>[2x]SEFVPPPECPVFEPSWEEFTDPLSFIGRIRPLAEKTGICKIRPPKDWQPPFACEVKSFRFTPRVQRLNELEAMTRVRLDFLDQLAKFWELQGSTLKIPVVERKILDLYALSKIVASKGGFEMVTKEKKWSKVGSRLGYLPGKGTGSLLKSHYERILYPYELFQSGVSLMG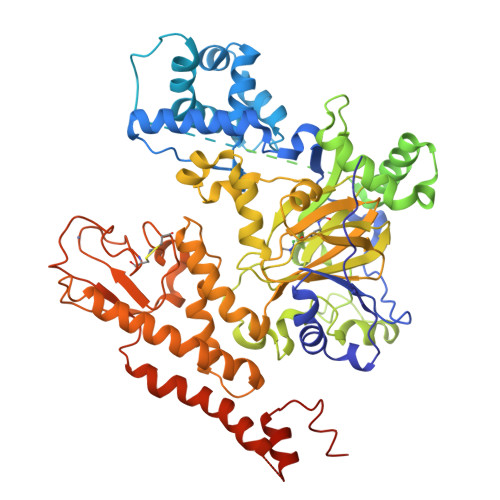VQMPNLDLKEKVEPEVLSTDTQTSPEPGTRMNILPKRTRRVKTQSESGDVSRNTELKKLQIFGAGPKVVGLAMGTKDKEDEVTRRRKVTNRSDAFNMQMRQRKGTLSVNFVDLYVCMFCGRGNNEDKLLLCDGCDDSYHTFCLIPPLPDVPKGDWRCPKCVAEECSKPREAFGFEQAVREYTLQSFGEMADNFKSDYFNMPVHMVPTELVEKEFWRLVSSIEEDVIVEYGADISSKDFGSGFPVKDGRRKILPEEEEYALSGWNLNNMPVLEQSVLAHINVDISGMKVPWLYVGMCFSSFCWHIEDHWSYSINYLHWGEPKTWYGVPSHAAEQLEEVMRELAPELFESQPDLLHQLVTIMNPNVLMEHGVPVYRTNQCAGEFVVTFPRAYHSGFNQGYNFAEAVNFCTADWLPIGRQCVNHYRRLRRHCVFSHEELIFKMAADPECLDVGLAAMVCKELTLMTEEETRLRESVVQMGVLMSEEEVFELVPDDERQCSACRTTCFLSALTCSCNPERLVCLYHPTDLCPCPMQKKCLRYRYPLEDLPSLLYGVKVRAQSYDTWVSRVTEALSANFNHKKDLIELRVMLEDAEDRKYPENDLFRKLRDAVKEAETCASVGNS> MIDITLPLTDIHRHLDGNIRAQTILDLGRQFNIALPAQTLETLIPHVQVTSTEPDLVSFLTK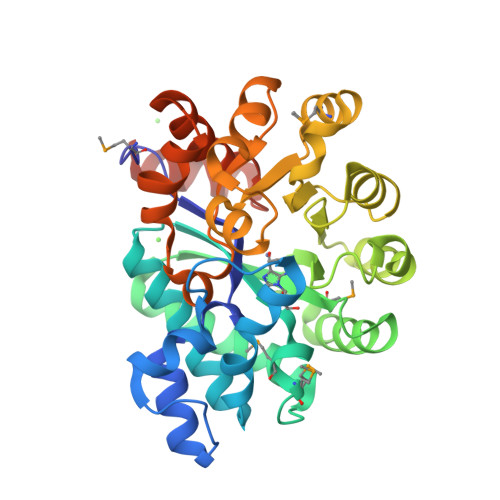LDWGVKVLASLDACRRVAFENIEDAARNGLHYVELRFSPGYMAMAHQLPIAGVVEAVIDGVRDGCNTFGVEARLIGIMSRTFGEAACLQELDALLAHRENITALDLAGDELGFPGSLFLSHFNRARDAGWHITVHAGEAAGPESIWQAIRELGAERIGHGVKAVEDRALMDFLAQQRIGIESCLTSNIQTSTVASLADHPLKTFLEHGVLASLNTDDPAVQGVDIIHEYHVAAPAAGLSREQIRQAQINGLEIAFLSDSEKRALREKVAEARGENLYFQ1-[(1H-benzimidazol-2-yl)methyl]-4-[(2,4-dichlorophenyl)methyl]-1,3-dihydro-2H-imidazol-2-one | C18 H14 Cl2 N4 O | 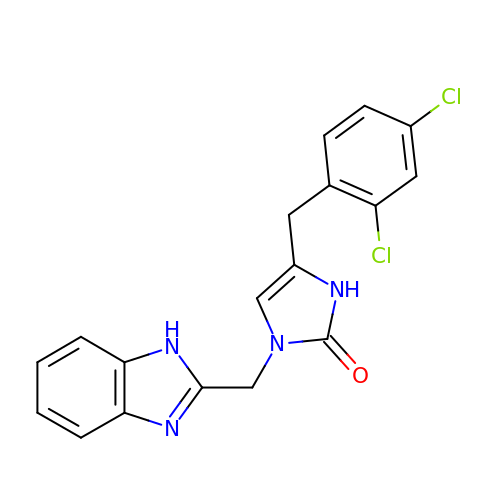ZHAMKWDXQMODPF-UHFFFAOYSA-N> MMLSLNNLQNIIYNPVIPFVGTIPDQLDPGTLIVIRGHVPSDADRFQVDLQNGSSVKPRADVAFHFNPRFKRAGCIVCNTLINEKWGREEITYDTPFKREKSFEIVIMVLKDKFQVAVNGKHTLLYGHRIGPEKIDTLGIYGKVN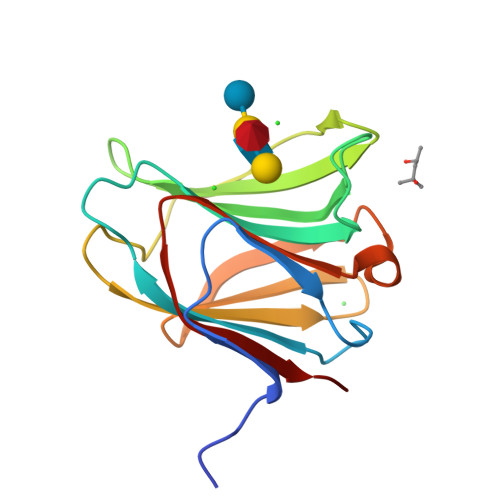IHSIGFSFS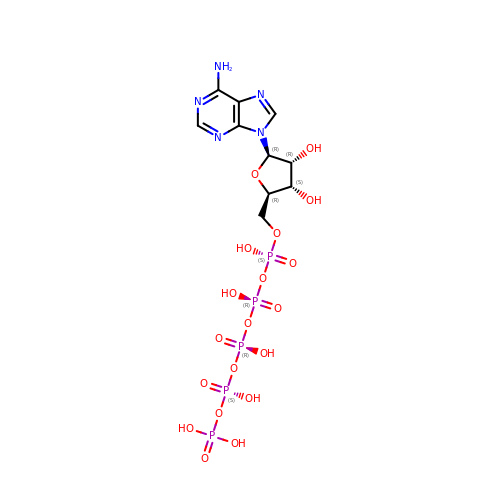ADENOSINE-5'-PENTAPHOSPHATE | C10 H18 N5 O19 P5 | WYJWVZZCMBUPSP-KQYNXXCUSA-N>MKIAVMTDSTSYLSQDLIDKYNIQIAPLSVTFDDGKNFTESNEIAIEEFYNKMASSQTIPTTSQPAIGEWITKYEMLRDQGYTDIIVICLSSGISGSYQSSYQAGEMVEGVNVHAFDSKLAAMIEGCYVLRAIEMVEEGYEPQQIIDDLTNMREHTGLYLIVDDLKNLQKSGRITGAQAWVGTLLKMKPVLKFEDGKIIPEEKVRTKKRAIQTLEKKVLDIVKDFEEVTLFVINGD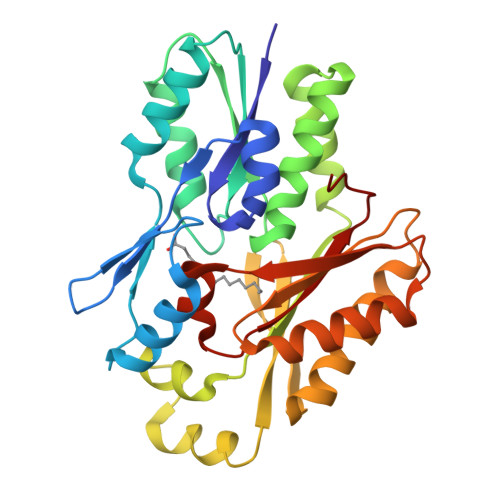HFEDGQALYKKLQDDCPSAYQVAYSEFGPVVAAHLGSGGLGLGYVGRKIRLT[2x]>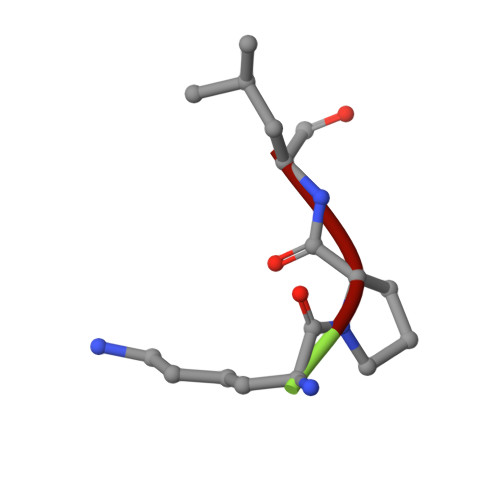 KPL> HHHHHHVAGAGAGENLYFQGMTVKSTLAVDMGGRYTGIFSYTTDSGFPKAKEARAYVLNMPDNDALTYSMAARTQTRHRIRSQQRFVLARRLTYILIEGKLKRKLSPREKEAISSLLRRRGYSRLESELDLSVLQGVESGFFKCFLPNFDEDENLLTQWTSLTDGYLQNNSDSRRQIQIFLESSKDSKEFLTVVKSQHQDTKEYKNALKVMRDDAESMIEQSMFGHKHRRLYLEAIAQDIPRDSRLKPIIEAFSGVEKFHHFIGNLSNLQLRALRWYFNDPSMKNNVFDKERLKSVLVRAYQFFHYPKDLTQQRAEVLNAYEGATDILETLQTLNPELTIPPYEDQNNRRPPLDQTLWLSPRLLDQRYGDTWEIWVQNLLRSPLS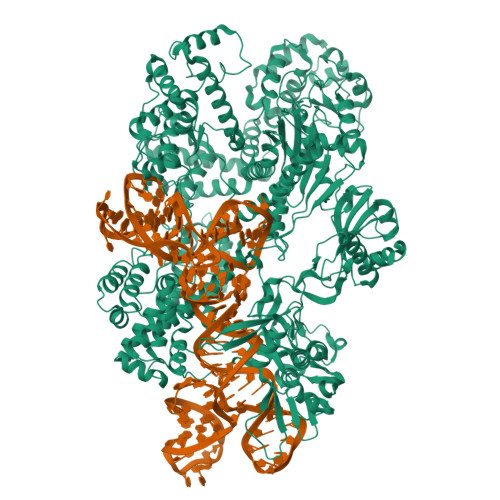KGIDENLDTILITTDRKARLLERQSGRLIHYTSQKLYHSYVLQRLLDRTVENDAYLLKTLVSSNRGNSNEIHQAQERLTRDLGSQHIKKFLDFVRQYYDEVDKAKRGLWFIVEKPLMERADIHPPMKNDSVILRLVGNILCVSDLVDLSFWTRKVKGQSTVRSLCTAIEKTRKEYGNSFNYLYQRALYLQSKGKKLSAEDKDFIKLQSNVLLVSDVIAEALDIKEEQKKKFANPFSLAQLYNIIETEKSGFISTTLAAVDENAWRNNLQGKARCVQLCADTVRPFDGALRNILDRQAYEIAKLKAEELLSTELKNQTIDLVVLLESNQFAFSASLAEVKKSANTAAIRQKVAKAQKRQQDRWLSKDERIKSASRGLCPYTGKNLGDKGEVDHIIPRSLSMNYMGSILNSEANLIYCSQEGNQLKLNGRKKLSDLADNYLKVVFGTADRGTICKYIEKSVSELTDAKIVQFELLDRSQQDAVRHALFLEDFSEARRRIIRLLGKINTARVNGTQAWFAKSFITKLRELTKEWCANNQITLAFDLYRLDAQTVSQDYRKKFALINKDWAKPDDKKQPIASHAIDAFCVFAAAKDKRNIANVLGVFDEVAEEQNLKTIAQLMPSEVNLISPKRKSILDKNEVGSRALMKEGIFAEHFLPILVRGDDCRIGFDWSESGSVKVKDADKLFGVLDGLLKQSQKRSVNGFETYTVDRIKAFELLHDVFIRPCSQKMLEQAEVLEKLHYITQNISVTSVYDAVNRQFKCREEILKDKDFDIKVDLGNRFGSAKGKITLPAKREWEKLVNRSELKNLIKDKLSDKGSEKTPDGETLIYDIFRSIPVQKLSHKATRRVWSLPKIPSISSGVRIKRKDSNGNDIYQLYMLNDTKCKGFVVNEKGVIDWSSDLVADLYKQPTLTILNGRYLKADQYVRMDQWYEVDCGRDDVIVKMCPGTSGRRYIEITQSKKQFEDWTGYISGSFWNYPVTIKLSSQQIANFVKNSQMPLLGKPRSGQITVITLGNTLKYWYCVESKNSMMNEAYQKAYLVHFNQKRPAAT> EVAAMDFTDKLIISRPLYISDNADPKCGYCNGKKDSSHKFASPGWSDFYKGDEDKVELQSSTVGFNSELVNAETYDKLCNLGFRRSGSFMYKTDMLRNCCRLYTIRTNEKYLTMSKELKTSLKRFKKKITSPEFKPQPKYVSWIDELCDYEPKSTSFKAVFEPAEFTDEKYDLYVRYQHYIHSDEDNTPSQFESFLCDTPFTDSEITGTEKEWE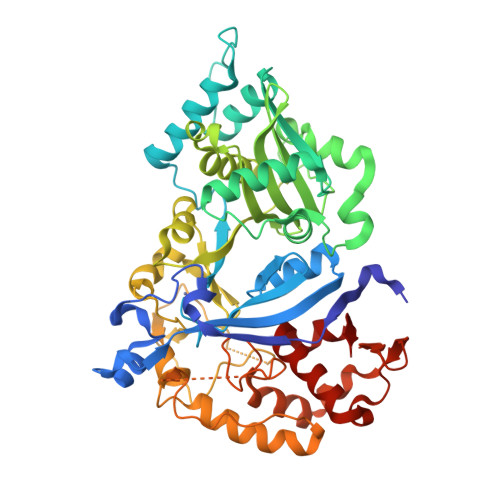QLNNWHNLQPGERVTKNGPAHECYYHNGKLIALSVLDFLPSGVSSVYFIWDPDYYDWSLGKVSALRELALVSKIGRPYYYLGYYIDDCPKMNYKAKFGGEILDVCNQKYVPLSKIHQIIKHNELFVGLNSTVASPDSEILITSASDKINFDEPFINAVDDIYGPNGNASQNAITSVAKLRKYGINYSPDLQRSIYKEIPNDGNSTSSASSDKKDVYRIPNVVPGLVPLMEIVSLFESGKMNELNNNVVLFDTKINALRIVRDFISEKPEIKTVITDVIRLIGLDNTKKAIIII ethyl 1-{(2S,3S)-3-[(3-{[(1R)-1-(4-fluorophenyl)ethyl]carbamoyl}-5-[methyl(methylsulfonyl)amino]benzoyl)amino]-2-hydroxy-4-phenylbutyl}-1H-pyrazole-4-carboxylate 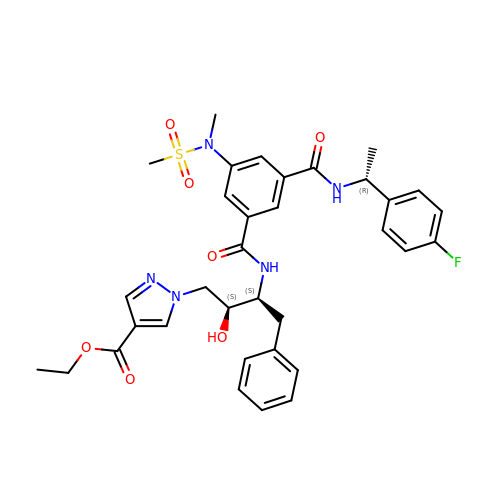| C34 H38 F N5 O7 S | MTFQLBNDNYIGHD-OJXBSAKDSA-N>[2x]GASMP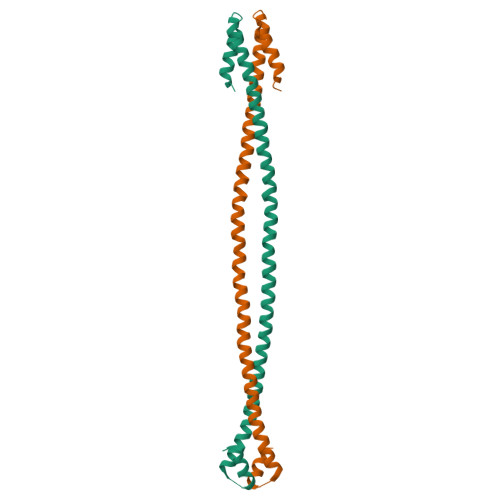LKPEEHEDILNKLLDPELAQSERTEALQQLRVNYGSFVSEYNDLTKSLSKANSEVAQWRTKYETDAIQRTEELEEAKKKLAQRLQEAEEAVEAVNAKCSSLEKTKHRLQNEIDFYFGKLRNIELICQENEGENDPVLQRIVDILYATDE> HHHHHHATAVVRCRTRLARRVVAAVGPDGLLPAPCESRVLESALALALLTEERAEADATARLTAYLRTTLRTAPPDPFQCAVARAVLGGAGERGERVGDEGDMDAGTALDAGLDGFDHFTAGRKRLMFRTVLAALGATGFPAVPWEAYDTRPQQSWLHMEMKALKVLAAHGTGHPDVVRDEDWRALLPALEPGPAWECNNLAQLLALLALRHSPRHRPALGDVLKHVAGRLRPDGGMPFIDGMTVFTTAAAGLALSLLPAPPACVTPMADALALRRNPDGGYGFHSGVAQSDVADTCYVLEFLRRAAPDRHRTAVAEAEGYLLALRNPDGGFPTFARGTSSEIAMTAAAASALAHDPDRREEVDEAVRYVVRHQRPDGTFERSWSRNAT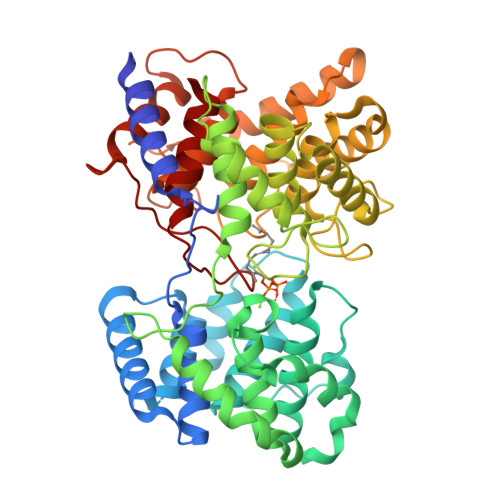NAVFRAVLALTGVAAHGEERRSRARAAERALAHLAATQNGDGGWGHAEAEPSDPISTAYAVIALARGPRARPGGPLDRALAYLVERQHPDGGYRSRPDQAGPRPLLYDVPALADVFVLLALAHAT Spermidine/spermine N-acetyltransferases (SSATs) are catabolic enzymes that acetylate polyamines and are critical for maintaining intracellular polyamine homeostasis. SpeG is an SSAT protein found in a variety of bacteria, including the human pathogen Vibrio cholerae. This protein adopts a dodecameric structure and contains an allosteric site, making it unique compared to other SSATs. The allosteric site is located between monomers that form the hexamers of the dodecamer, and some evidence has been provided that shows when polyamine binds to these sites, the dodecamer tightens.

R1C1 replaces all residues of this region with the hSSAT1 protein sequence, R1C2 replaces the first half of the residues, R1C3 replaces the first three quarters of the residues, and R1C4 replaces the latter half of the residues of this region. Despite crystallizing in a range of crystallography space groups, six structures adopted the apo-conformation of VcSpeG. Minor differences in residue positions were observed in the overlaid R1C2 (K23-E29) and R3C1 (R149, L150, F151, K152) crystal structures and models. On the other hand, only substituting the first eight residues of this loop (R1C2) caused a minimal (1.7-fold) decrease in activity compared to WT. Based on the kinetic results, it became clear that the region of the allosteric loop that was critical for activity was between residues 31–34 (WFEE). In the WT structure, this portion of the allosteric loop forms several important interactions, including an NH-arene interaction between Q86 and W31, π-π interactions between F32 of Region 1 and F149 of Region 3, an H-bond between the terminal amine of spm and the sidechain of E33 in the allosteric site, and a hydrophobic interaction between E34 and the methylenes of spm in the allosteric site. The R1C1, R1C3, and R1C4 constructs all have MEEQ in place of WFEE, which would disrupt these interactions and may explain the reduced activity of these constructs. On the other hand, the R1C2 construct retained these residues and may explain why this construct retained activity. The investigation of alterations to Region 1 of the VcSpeG protein (R1C1-R1C4) showed we could replace residues in the first half of the allosteric loop (R1C2) and retain moderate activity, but exchanging residues in either the second half of the loop (R1C4), the first three quarters of the loop (R1C3) or the entire loop (R1C1) caused the enzyme to be inactive. Since the R1C2 construct still maintained significant activity, it appears retention of acidity in the allosteric site may enable polyamine binding and subsequent catalysis, especially when significant van der Waals and complementary electrostatic interactions between Regions 1 and 3 were maintained.

>[12x]MNSQLTLRALERGDLRFIHNLNKELARYEYWFEEPYESFDELEELYNKHIHDNAERRFVVEDAQKNLIGLVELIEINYIHRSAEFQIIIAPEHQGKGFARTLINRALDYSFTILNLHKIYLHVAVENPKAVHLYEECGFVEEGHLVEEFFINGRYQDVKRMYILQSKYLNRSE(S)-MANDELIC ACID NITRILE | C8 H7 N O | 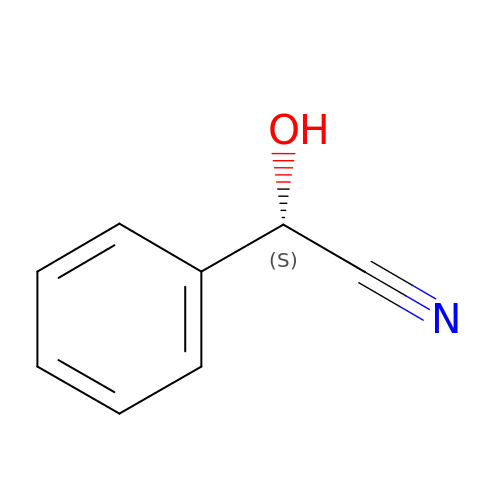NNICRUQPODTGRU-MRVPVSSYSA-N>MHTQVHTARLVHTADLDSETRQDIRQMVTGAFAGDFTETDWEHTLGGMHALIWHHGAIIAHAAVIQRRLIYRGNALRCGYVEGVAVRADWRGQRLVSALLDAVEQVMRGAYQLGALSSSARARRLYASRGW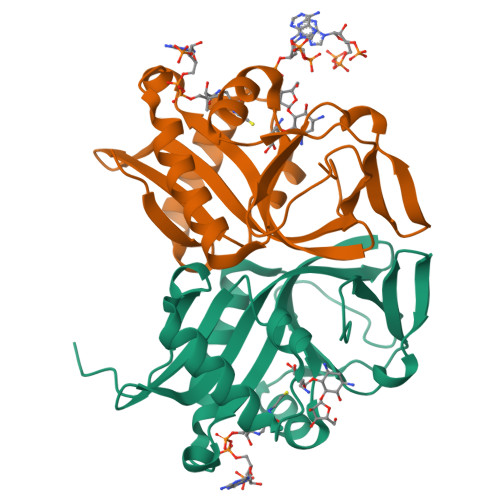LPWHGPTSVLAPTGPVRTPDDDGTVFVLPIDISLDTSAELMCDWRAGDVW[2x]> IVYP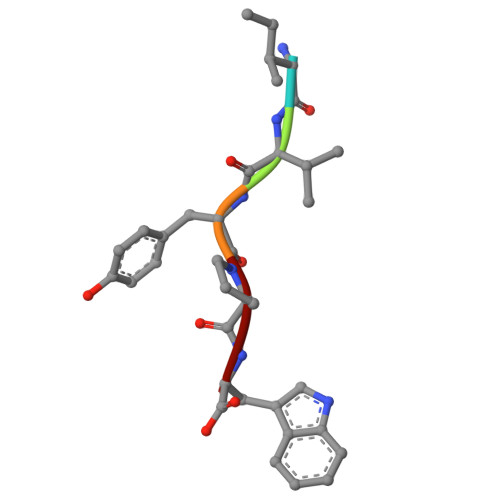W> GLHSWGSEMDLVDSLDNPDEIQDNEEIQTQNVEAAQGEELATEVGLRATENDGSLSEQLNMSQPMFLNFKKHKVNIYAATHTKVDHIFGRAWAVGVFNTETAAIQKFDLHFPTSTHGALSRFFCHWTGELNIHILNVSTTNAFLKVAHTWFGTDSGIARTATLESNGTMIIPPNEQMTLCVPYYSEVPLRCVKGSDRNSAGLGSLFTQAVGRTISNRVQIFVSFRCPNFFFPL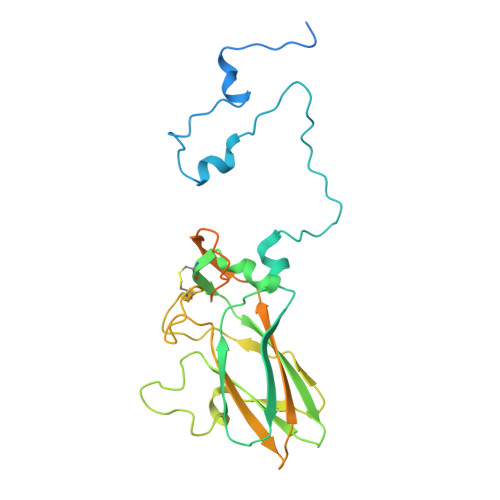PAPREATSASILERVDEANAEELEAVLEARTPDAPLRLKFNPEDPLKQLREAAKAYFNIMHSDE> MMKKIDVKILDPRVGKEFPLPTYATSGSAGLDLRACLNDAVELAPGDTTLVPTGLAIHIADPSLAAMMLPRSGLGHKHGIVLGNLVGLINSDYQGQLMISVWNRGQDSFTIQPGERIAQMIFVPVVQAEFNLVEDFDATDRGEGG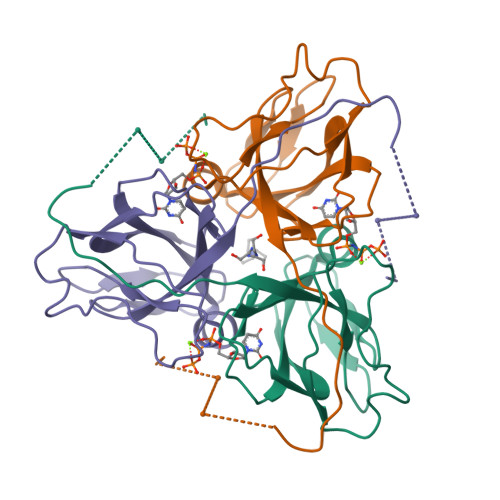FGHSGRQ>GEFMAAERGAGQQQSQEMMEVDRRVESEESGDEEGKKHSSGIVADLSEQSLKDGEERGEEDPEEEHELPVDMETINLDRDAEDVDLNHYRIGKIEGFEVLKKVKTLCLRQNLIKCIENLEELQSLRELDLYDNQIKKIENLEALTELEILDISFNLLRNIEGVDKLTRLKKLFLVNNKISKIENLSNLHQLQMLELGSNRIRAIENIDTLTNLESLFLGKNKITKLQNLDALTNLTVLSMQSNRLTKIEGLQNLVNLRELYLSHNGIEVIEGLENNNKLTMLDIASNRIKKIENISHLTELQEFWMNDNLLESWSDLDELKGARSLETVYLERNPLQKDPQYRRKVMLALPSV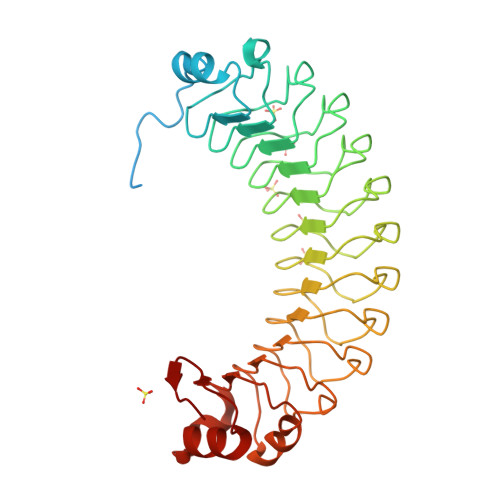RQIDATFVRF[5x]N~5~-[(E)-imino(methylsulfanyl)methyl]-L-ornithine | C7 H15 N3 O2 S 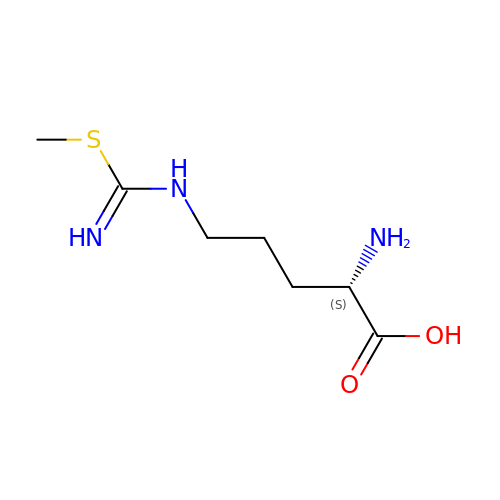| NGVMVBQRKZPFLB-YFKPBYRVSA-N>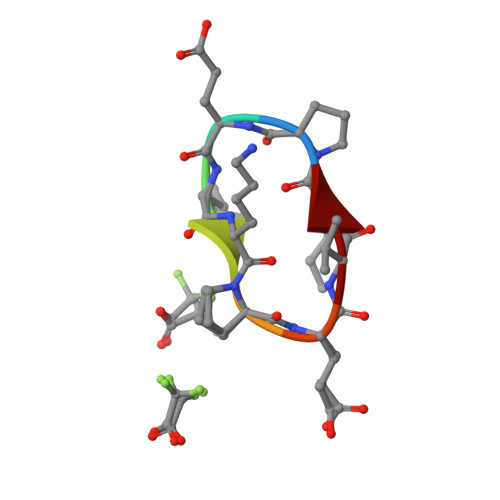 PEVKPEVK> MELTPREKDKLLLFTAALVAERRLARGLKLNYPESVALISAFIMEGARDGKSVASLMEEGRHVLTREQVMEGVPEMIPDIQVEATFPDGSKLVTVHNPII;> MIPGEYHVKPG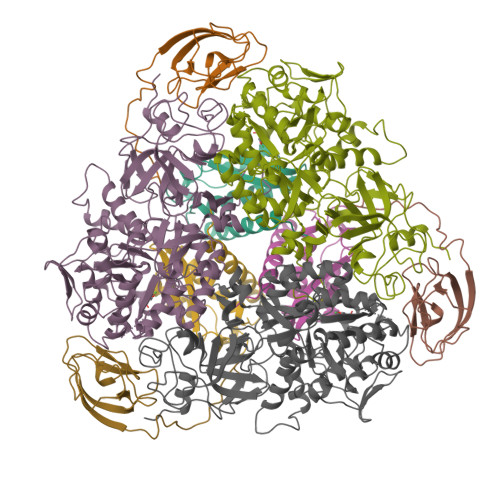QIALNTGRATCRVVVENHGDRPIQVGSHYHFAEVNPALKFDRQQAAGYRLNIPAGTAVRFEPGQKREVELVAFAGHRAVFGFRGEVMGPLEVNDE;> MSNISRQAYADMFGPTVGDKVRLADTELWIEVEDDLTTYGEEVKFGGGKVIRDGMGQGQMLAADCVDLVLTNALIVDHWGIVKADIGVKDGRIFAIGKAGNPDIQPNVTIPIGAATEVIAAEGKIVTAGGIDTHIHWICPQQAEEALVSGVTTMVGGGTGPAAGTHATTCTPGPWYISRMLQAADSLPVNIGLLGKGNVSQPDALREQVAAGVIGLKIHEDWGATPAAIDCALTVADEMDIQVALHSDTLNESGFVEDTLAAIGGRTIHTFHTEGAGGGHAPDIITACAHPNILPSSTNPTLPYTLNTIDEHLDMLMVDHHLDPDIAEDVAFAESRIRRETIAAEDVLHDLGAFSLTSSDSQAMGRVGEVILRTWQVAHRMKVQRGALAEETGDNDNFRVKRYIAKYTINPALTHGIAHEVGSIEVGKLADLVVWSPAFFGVKPATVIKGGMIAIAPMGDINASIPTPQPVHYRPMFGALGSARHHCRLTFLSQAAAANGVAERLNLRSAIAVVKGCRTVQKADMVHNSLQPNITVDAQTYEVRVDGELITSEPADVLPMAQRYFLF>LPSLEDLLFYTIAEGQEKIPVHKFITALKSTGLRTSDPRLKECMDMLRLTLQTTSDGVMLDKDLFKKCVQSNIVLLTQAFRRKFVIPDFMSFTSHIDELYESAKKQSGGKVADYIPQLAKFSPDLWGVSVCTVDGQRHSIGDTKVPFCLQSCVKPLKYAIAVNDLGTEYVHRYVGKEPSGLRFNKLFLNEDDKPHNPMVNAGAIVVTSLIKQGVNNAEKFDYVMQFLNKMAGNEYVGFSNATFQSERESGKRNFAIGYYLKEKKCFPEGTDMVGILDFYFQLCSIEVTCESASVMAATLANGGFCPITGERVLSPEAVRNTLSLMHSCGMYDFSGQFAFHVGLPAKSGVAGGILLVVPNVMGMMCWSPPLDKMGNSVKGIHFCHDLVSLCNFHNYDN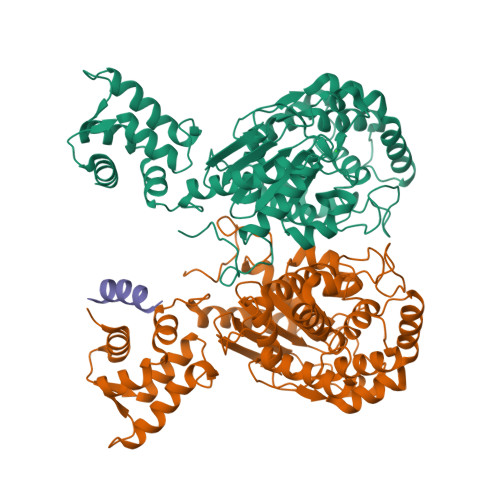LRHFAKKLDPRREG[2x];> AKGALQELGAGLTA>SVDC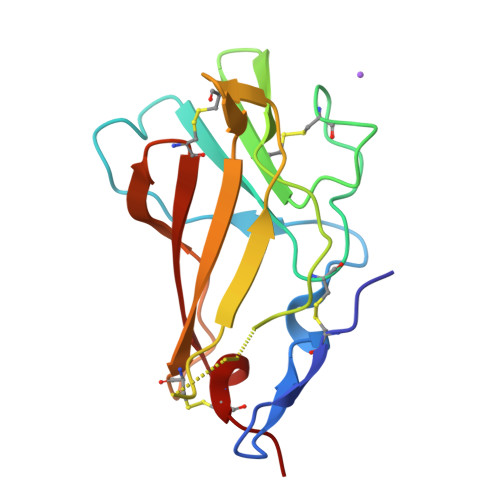QVTDLAGNEYDLTGLSTVRKPWTAVDTSVDGRKRTFYLSVCNPLPYIPGCQGSAVGSCLVSEGNSWNLGVVQMSPQAAANGSLSIMYVNGDKCGNQRFSTRITFECAQISGSPAFQLQDGCEYVFIWRTVEACPVV[2x]>UUGCGUCACCUCGAGCAAGUCGC[3x];> GCGUCACCU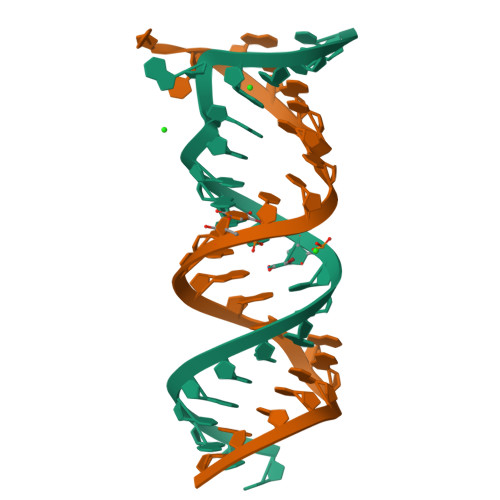CGAGCAAGUCGC> MSLQGIHLSDLSYKHAILKESQYTIKRDVGTTTAVTPSSLQQEITLLCGEILYAKHADYKYAAEIGIQYISTALGSERVQQILRNSGSEVQVVLTRTYSLGKIKNNKGEDLQMLDIHGVEKSWVEEIDKEARKTMATLLKESSGNIPQNQRPSAPDTPIILLCVGALIFTKLASTIEVGLETTVRRANRVLSDALKRY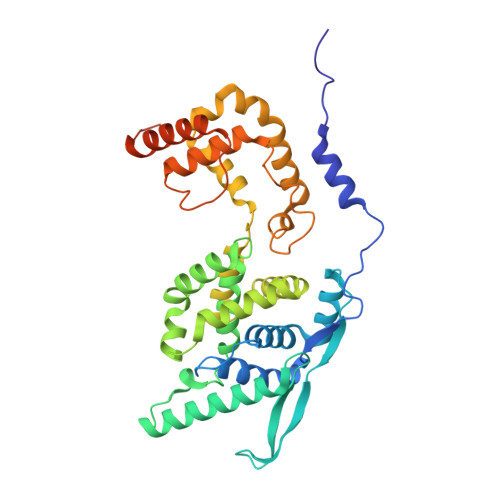PRMDIPKIARSFYDLFEQKVYHRSLFIEYGKALGSSSTGSKAESLFVNIFMQAYGAGQTMLRWGVIARSSNNIMLGHVSVQAELKQVTEVYDLVREMGPESGLLHLRQSPKAGLLSLANCPNFASVVLGNASGLGIIGMYRGRVPNTELFSAAESYAKSLKESNKINFSSLGLTDEEKEAAEHFLNVSDDSQNDYE> MDLADRFAELERRYDARLGVYVPATGTTAAIEYRADERFAFCATFKAPLVAAVLHQNPLTHLDKLITYTSDDIRSISPVAQQHVQTGMTIGQLCDAAIRYSDGTAANLLLADLGGPGGGTAAFTGYLRSLGDTVSRLDAEEPELNRDPPGDERDTTTPHAIALVLQQLVLGNALPPDKRALLTDWMARNTTGAK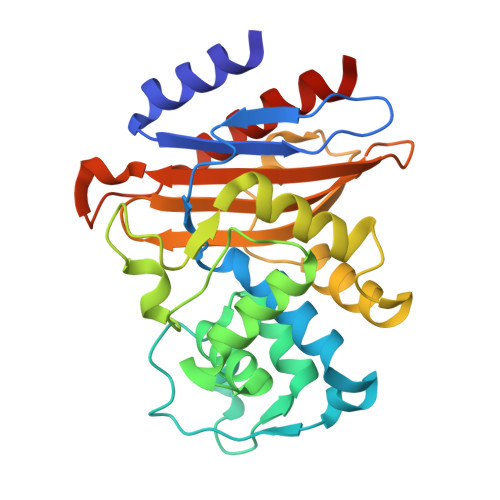RIRAGFPADWKVIDKTGTGDYGRANDIAVVWSPTGVPYVVAVMSDRAGGGYDAEPREALLAEAATCVAGVLALEHHHHHH>[2x]MGWSCIILFLVATATGVHSGGWSHPQFEKAEAAAKEAAAKEAAAKAAVAEMNPNVNVFVPPRDGFSGPAPRKSKLICEATNFTPKPITVSWLKDGKLVESGFTTDPVTIENKGSTPQTYKVISTLTISEIDWLNLNVYTCRVDHRGLTFLKNVSSTCAASPSTDILTFTIPPSFADIFLSKSANLTCLVSNLATYETLNISWASQSGEPLETKIKIMESHPNGTFSAKGVASVCVEDWNNRKEFVCTVTHRDLPSPQKKFISKPNEVHKHPPAVYLLPPAREQLNLRESATVTCLVKGFSPADISVQWLQRGQLLPQEKYVTSAPMPEPGAPGFYFTHSILTVTEEEWNSGETYTCVVGHEALPHLVTERTVDKSTEGEVNAEEEGFENLWTTASTFIVLFLLSLFYSTTVTLFKVK;> DYKDDDDKMPGGLEALRALPLLLFLSYACLGPGCQALRVEGGPPSLTVNLGEEARLTCENNGRNPNITWWFSLQSNITWPPVPLGPGQGTTGQLFFPEVNKNHRGLYWCQVIENNILKRSCGTYLRVRNPVPRPFLDMGEGTKNRIITAEGIILLFCAVVPGTLLLFRKRWQNEKFGRSIATRSMFKGIVEGIGIIEKIDIYTDLDKYAIRFPENMLNGIKKESSIMFNGCFLTVTSVNSNIVWFDIFEKEARKLDTFREYKVGDRVNLGTFPKFGAASGGHILSARISCVASIIEIIENEDYQQMWIQIPENFTEFLIDKDYIAVDGISLTIDTIKNNQFFISLPLKIAQNTNMKWRKKGDKVNVELSNKINANQCW;> MATLVLSSMPCHWLLFLLLLFSGEPVPAMTSSDLP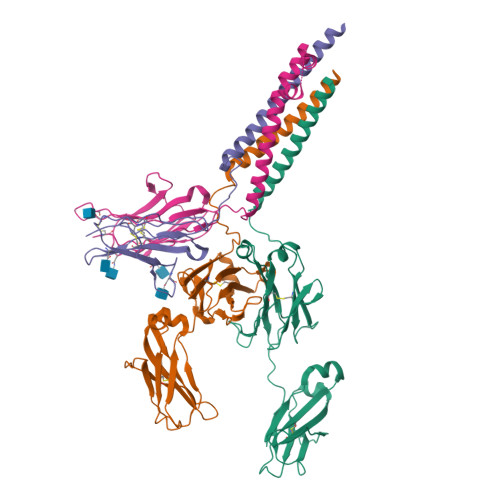LNFQGSPCSQIWQHPRFAAKKRSSMVKFHCYTNHSGALTWFRKRGSQQPQELVSEEGRIVQTQNGSVYTLTIQNIQYEDNGIYFCKQKCDSANHNVTDSCGTELLVLGFSTLDQLKRRNTLKDGIILIQTLLIILFIIVPIFLLLDKDDGKAGMEEDHTYEGLNIDQTATYEDIVTLRTGEVKWSVGEHPGQE>MLWKKTFTLENLNQLCSNSAVSHLGIEISAFGEDWIEATMPVDHRTMQPFGVLHGGVSVALAETIGSLAGSLCLEEGKTVVGLDINANHLRPVRSGKVTARATPINLGRNIQVWQIDIRTEENKLCCVSRLTLSVINLLEHHHHHH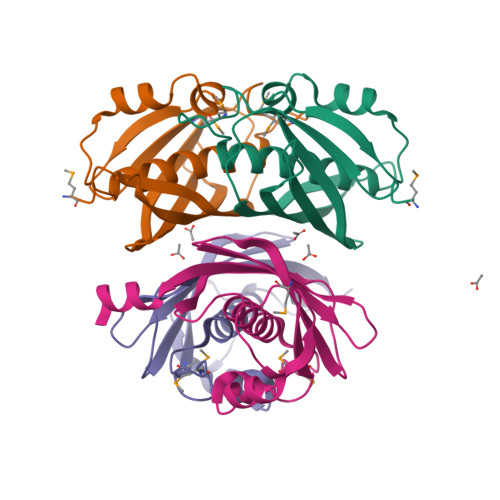[8x]3-(3-methoxyphenyl)benzoic 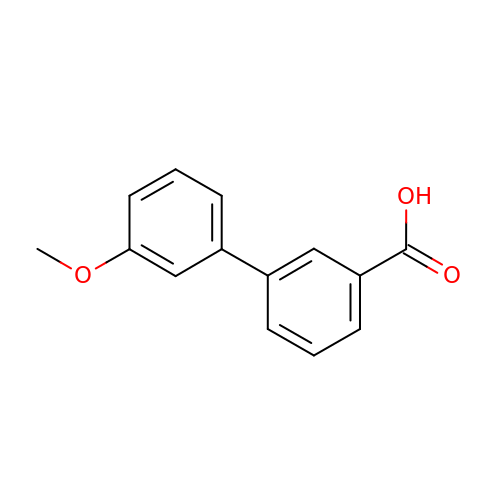acid | C14 H12 O3 | JFPVSZXZHHOWMI-UHFFFAOYSA-N> RIA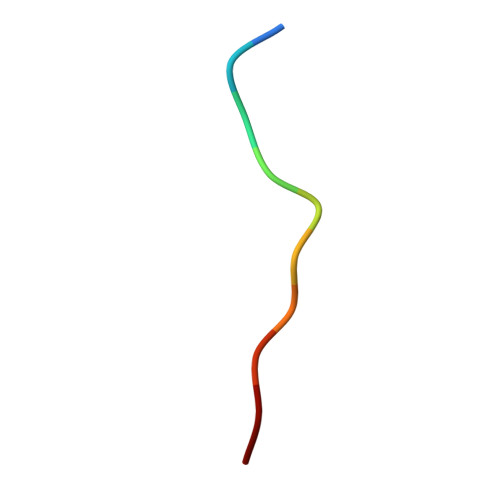CEEEFSD5A,6-ANHYDROTETRACYCLINE | C22 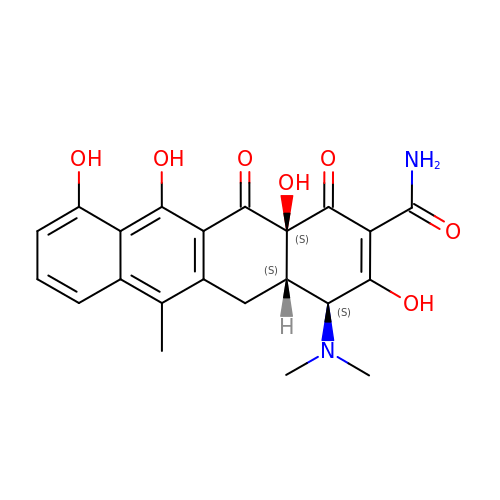H22 N2 O7 | CXCVEERYMJZMMM-DOCRCCHOSA-N The androgen receptor (AR) is the cellular mediator of the actions of the hormone 5-α dihydrotestosterone (DHT). Androgen binding to AR leads to activation of genes involved in the development and maintenance of the male reproductive system and other tissues such as bone and muscle. AR is distinguished from other nuclear receptors in that after hormone binding, it preferentially responds to a specialized set of coactivators bearing aromatic-rich motifs, while responding poorly to coactivators bearing the leucine-rich “NR box” motifs favored by other nuclear receptors. Structures of AR in complex with FxxLF, LxxLL, FxxLW, WxxLF, WxxVW, FxxFF, and FxxYF motifs reveal a changing surface of the AR coactivator binding interface that permits accommodation of both AR-specific aromatic-rich motifs and canonical leucine-rich motifs.

To understand how the AR AF-2 accommodates tryptophan residues, structures of AR in complex with peptides containing tryptophan substitutions at the +1 or +5 position, or both, were determined. In FxxLW and WxxVW, the −2 serine forms a bidentate hydrogen-bonding interaction, making hydrogen bonds to both Glu897 and the backbone amide group of the +2 residue. Thus, tryptophan substitutions are tolerated, but they induce a shift in the peptide backbone that precludes interactions with one of the charge clamp residues. This suboptimal interaction is compensated partially by interactions of flanking residues with the AR surface. In contrast, the +5 indole group of FxxLW is rotated almost 90°, resulting in burial of both rings of the indole group, as well as the formation of a strong hydrogen bond between the indole nitrogen and Gln730. Binding in this orientation appears to be highly favorable, as the FxxLW peptide deviates from helical geometry at the +5 position to do so. The equilibrium dissociation constants (Kd) were directly determined for the interaction between the AR LBD and FxxLF and LxxLL peptides and one variant tryptophan-containing peptide, FxxLW, using surface plasmon resonance. Surprisingly, the affinity of FxxLW, with a Kd of 920 nM, was slightly better than FxxLF, in spite of the presence of the tryptophan residue at the +5 position.

> GSPGISGGGGGSHIEGYECQPIFLNVLEAIEPGVVCAGHDNNQPDSFAALLSSLNELGERQLVHVVKWAKALPGFRNLHVDDQMAVIQYSWMGLMVFAMGWRSFTNVNSRMLYFAPDLVFNEYRMHKSRMYSQCVRMRHLSQEFGWLQITPQEFLCMKALLLFSIIPVDGLKNQKFFDELRMNYIKELDRIIACKRKNPTSCSRRFYQLTKLLDSVQPIARELHQFTFDLLIKSHMVSVDFPEMMAEIISVQVPKILSGKVKPIYFHTQ;> SSKFAALWDPPKLSRSGSGK> MFQKQVYRQYTPGFPGDLIEDGPKRARPGRIMSLSAVNPAATATGPNRISRAFGYAGDVSALGEGQPKTIAARASEVVIGGANFFGVLGHPKHYALFGSAGDSLAPSYDLPDGAEGEFFDMATGLVVEIFNGAATALDLDYGDLVAYVPNNLPTADNA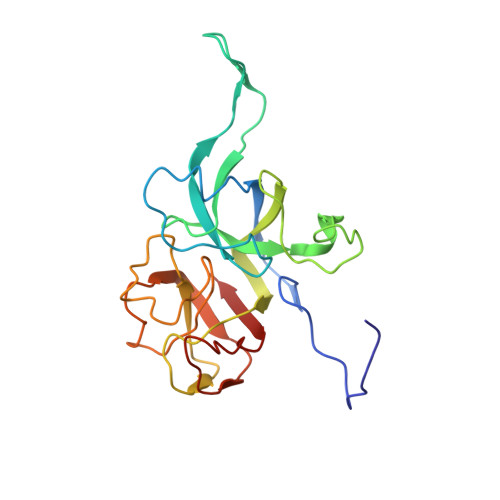LGLPAGALVGFKAGSMPTGLVQIPNARIVNAISLPAQSAGNLVAGVTIVQLTQ> MAFKRAIIFTSFNGFEKVSRTEKRRLAKIINARVSIIDEYLRAKDTNASLDGQYRAFLFNDESPAMTEFLAKLKAFAESCTGISIDAWEIEESEYVRLP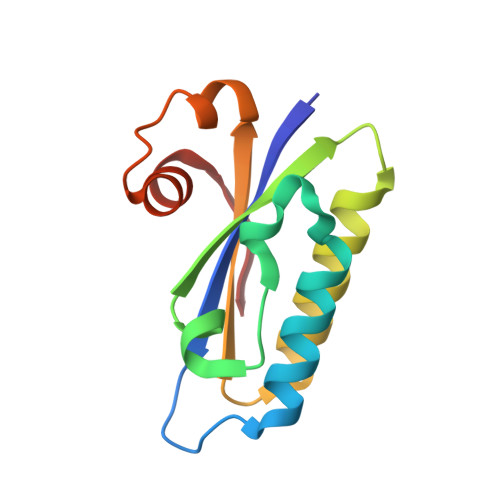VERRDFLAAANGKEIFKI> HPICEVSKVASHLEVNCDKRQLTALPPDLPKDTTILHLSENLLYTFSLATLMPYTRLTQLNLDRCELTKLQVDGTLPVLGTLDLSHNQLQSLPLLGQTLPALTVLDVSFNRLTSLPLGALRGLGELQELYLKGNE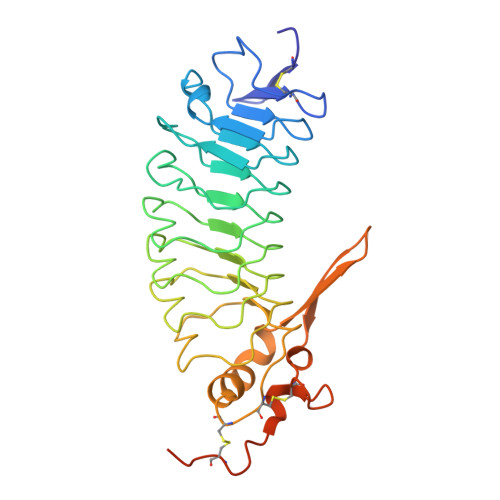LKTLPPGLLTPTPKLEKLSLANNQLTELPAGLLNGLENLDTLLLQENSLYTIPKGFFGSHLLPFAFLHGNPWLCNCEILYFRRWLQDNAENVYVWKQGVDVKAVTSNVASVQCDNSDKFPVYKYPGKGCPTLGDEGDTDLYDYYPEEDTEGDKVR>[2x]MSQSGEDLHSPTYLSWRKLQLSRAKLKASS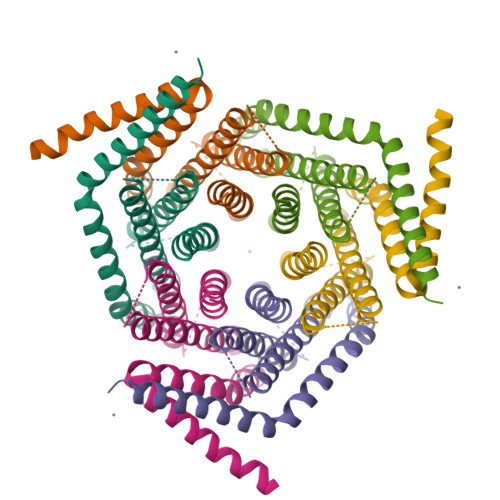WTSALLSGFAMVAMVEVQLDHDTNVPPGMLIAFAICTTLLVAVHMLALMISTCILPNIETVSNLHSISLVHESPHERLHWYIETAWAFSTLLGLILFLLEIAILCWVKFYDLSRRAAWSATVVLIPVMIIFMAFAIHFYRSLVSHKYEVTVSGIRELEMLKEQMEQDHLEHHNNIRNNGEGEEF The outer surface of the head is decorated with the highly antigenic outer capsid protein Hoc and the small outer capsid protein Soc. The 376-residue Hoc is a monomeric fiber consisting of a string of four domains connected by flexible short linkers, of which the three N-terminal domains have an immunoglobulin (Ig)-like fold. The Hoc subunits bind near the centers of gp23* capsomers, one per hexon, and have only a marginal effect on the capsid stability. Each T4-Hoc fiber attaches randomly to the center of gp23* hexameric capsomers in one of the six possible orientations, though at the vertex-proximal hexamers that deviate from 6-fold symmetry, Hoc binds in two preferred orientations related by 180° rotation.

However, fitting of the Hoc C-terminal domain (residues 281–376) from the AlphaFold model into the cryo-EM maps at the vertex-proximal gp23* capsomers of the isometric and prolate capsids showed only two preferred orientations for the bound Hoc molecules. These two preferred orientations, which gave major contributions to the observed cryo-EM density, are related by 180° rotation around the hexamer axis. The Hoc chains fitted into the density corresponding to the two preferred orientations showed significant overlap, indicating that only one chain can bind to the center of the gp23* hexamer. The 3.4 Å-resolution five-fold-symmetric reconstruction of the native prolate T4 capsid (EMDB-32109) also shows similar preferred orientations to the Hoc C-terminal domains attached to the vertex-proximal gp23* hexamers. Similar fitting and refinement procedures were performed for the Hoc C-terminal domain attached in the two preferred orientations to the gp23* hexamer adjacent to the “top” pentameric vertex of the prolate capsid located on the five-fold symmetry axis. The occupancy values for the two orientations of Hoc were 0.42 and 0.35, which are close to those in the isometric head. The Hoc C-terminal domain, in both the preferred orientations, interacts with six gp23* subunits with an interface area of ~1200 Å2. However, at the gp23* hexamers proximal to the capsid vertices, which deviate from the six-fold symmetry, Hoc binds in two preferred orientations, which are related by 180° rotation, in part because the other orientations involve clashes and, most likely, less stable interactions.

>AEIGGDHGYNATNIAAGQTSGAVTQIGPAVMGMVRRAIPNLIAFDICGVQPMNSPTGQVFALRAVYGKDPVAAGAKEAFHPMYGPDAMFSGQGAAKKFPALAASTQTTVGDIYTHFFQETGTVYLQASVQVTIDAGATDAAKLDAEIKKQMEAGALVEIAEGMATSIAELQEGFNGSTDNPWNEMGFRIDKQVIEAKSRQLKAAYSIELAQDLRAVHGMDADAELSGILATEIMLEINREVVDWINYSAQVGKSGMTLTPGSKAGVFDFQDPIDIRGARWAGESFKALLFQIDKEAVEIARQTGRGEGNFIIASRNVVNVLASVDTGISYAAQGLATGFSTDTTKSVFAGVLGGKYRVYIDQYAKQDYFTVGYKGPNEMDAGIYYAPYVALTPLRGSDPKNFQPVMGFKTRYGIGINPFAESAAQAPASRIQSGMPSILNSLGKNAYFRRVYVKGI[6x];>[2x]MTFTVDITPKTPTGVIDETKQFTATPSGQTGGGTITYAWSVDNVPQDGAEATFSYVLKGPAGQKTIKVVATNTLSEGGPETAEATTTITVKNKTQTTTLAVTPASPAAGVIGTPVQFTAALASQPDGASATYQWYVDDSQVGGETNSTFSYTPTTSGVKRIKCVAQVTATDYDALSVTSNEVSLTVNKKTMNPQVTLTPPSINVQQDASATFTANVTGAPEEAQITYSWKKDSSPVEGSTNVYTVDTSSVGSQTIEVTATVTAADYNPVTVTKTGNVTVTAKVAPEPEGELPYVHPLPHRSSAYIWCGWWVMDEIQKMTEEGKDWKTDDPDSKYYLHRYTLQKMMKDYPEVDVQESRNGYIIHKTALETGIIYTYP2-(butanoylamino)-2-deoxy-beta-D-glucopyranose | C10 H19 N O6 | 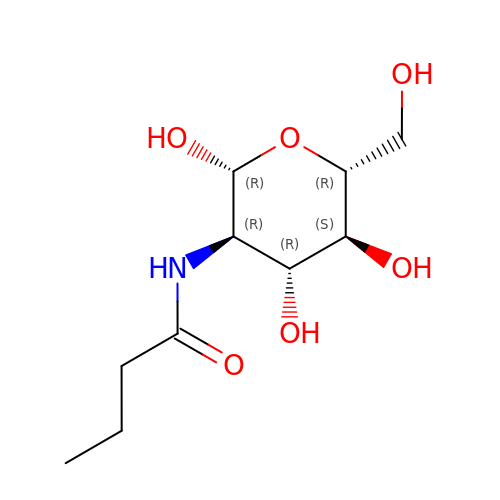RPJMPMDUKSRLLF-QXOHVQIXSA-N>GAM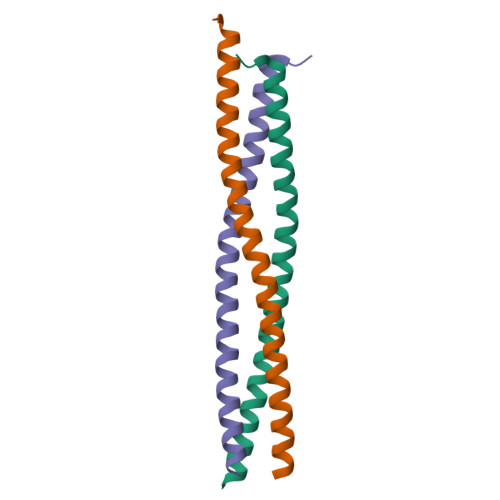AEAEAEVTLRELQEALEEEVLTRQSLSREMEAIRTDNQNFASQLREAEARNRDLEAHVRQLQERMELLQAEGATAVTG[3x]>[2x]MPIAKVHRIATASPDDVSGLAAAIATGAIAPAGILAIFGKTEGNGCVNDFSRGFAVQSLQMLLRGHMGAAADEVCLVMSGGTEGGMSPHFLVFERAEGNAPEAAPALAIGRAHTPDLPFEALGRMGQVRMVAQAVRRAMAAAGITDPEDVHFVQVKCPLLTAMRVKEAEARGATTATSDTLKSMGLSRGASALGIALALGEVAEDALSDAVICADYGLWSARASCSSGIELLGHEIVVLGMSEGWSGPLAIAHGVMADAIDVTPVKAALSALGAEAGEATIVLAKAEPSRSGRIRGKRHTMLDDSDISPTRHARAFVAGALAGVVGHTEIYVSGGGEHQGPDGGGPVAVIAARTMG

The first step of cyanuric acid metabolism is catalyzed by cyanuric acid hydrolase (CAH) and results in s-triazine ring opening to produce unstable carboxybiuret, which undergoes rapid, spontaneous decarboxylation to yield biuret. We have conducted X-ray crystallographic studies of the cyanuric acid hydrolase from Azorhizobium caulinodans ORS 571 (NCBI reference sequence; YP_001526808.1), denoted here as CAH. AtzD and CAH are 51% identical in a pairwise amino acid sequence alignment and share an overall unique fold consisting of three structurally analogous domains that form a barrel structure. The active site of CAH with the pseudo 3-fold rotational symmetry constructed from 3 structurally homologous domains seems optimal for catalyzing hydrolysis of the 3-fold symmetrical cyanuric acid.

The crystal structure determination of a selenomethionine substituted CAH-inhibitor complex was accomplished using the single wavelength anomalous diffraction (SAD) phasing. The final 2.7 Å resolution model revealed a protein fold consisting of a β-barrel-like core with α helices organized on the outside, forming a central cavity ∼10 Å wide at its opening. In the CAH-barbituric acid complex crystal, the asymmetric unit contains a dimer related by a non-crystallographic two-fold axis that further dimerizes via a crystallographic two-fold axis to form a tetramer with 222 point symmetry. The structure of the CAH monomer exhibits an internal pseudo-three fold symmetry, consistent with our preliminary analyses of the X-ray diffraction data. In both subunits in the asymmetric unit of the CAH-barbituric acid complex crystal, a molecule of the highly analogous substrate analog, barbituric acid was found at one end of the barrel structure, unambiguously identifying the location of the active site and the mode of substrate-binding. In addition, another barbituric acid molecule, albeit at lower occupancy, was observed on the surface of one of the CAH subunits near the opening of the potential substrate channel, which is discussed later in more detail. A highly organized, trimeric conglomeration of serines, lysines, and arginines surrounds the bound barbituric acid, mirroring the three-fold symmetrical shape of the substrate. Three serine residues (Ser79, Ser226, Ser333) lie in close proximity to the carbonyl carbons of barbituric acid, suggesting that one could act as the nucleophile in a nucleophilic attack on the substrate. The combination of distance and BD angles data indicate that Ser226 is the most likely nucleophile of the three serines in the CAH active site.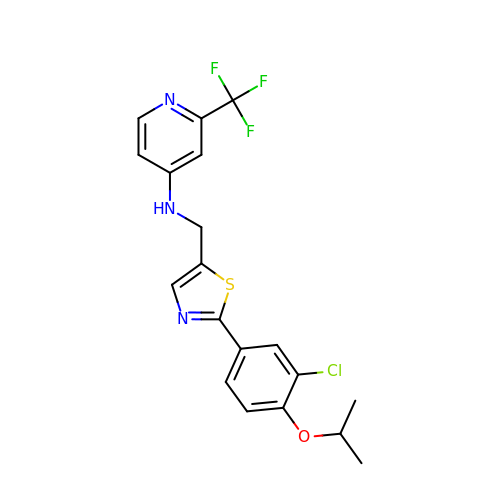~{N}-[[2-(3-chloranyl-4-propan-2-yloxy-phenyl)-1,3-thiazol-5-yl]methyl]-2-(trifluoromethyl)pyridin-4-amine | C19 H17 Cl F3 N3 O S | GQVXDNRONWTUJQ-UHFFFAOYSA-N> MAFISSGYNPEKPMANRITDIGPRKFDEFFPPVIAKNFGSWLYHEILEPGVLMHVAESGDKVYTVRVGAARLMSITHIREMCDIADKYCGGHLRFTTRNNVEFMVADEASLKALKEDLASRKFDGGSLKFPIGGTGAGVSNIVHTQGWVHCHTPATDASGPVKAIMDEVFEDFQSMRLPAPVRISLACCINMCGAVHCSDIGVVGIHRKPPMIDHEWTDQLCEIPLAVASCPTAAVRPTKLEIGDKKVNTIAIKNERCMYCGNCYTMCPALPISDGEGDGVVIMVGGKVSNRISMPKFSKVVVAYIPNEPPRWPSLTKTIKHIIEVYSANAYKYERLGEWAERIGWERFFSLTG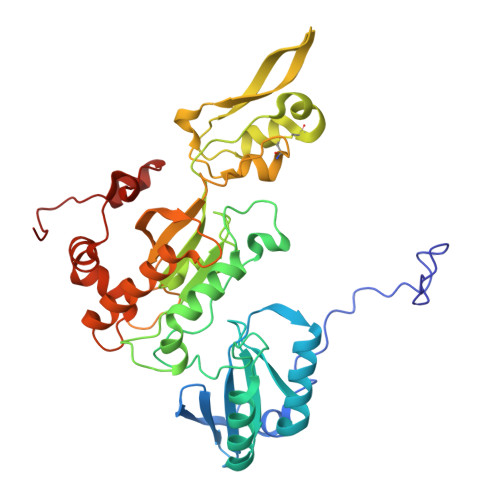LEFSHHLIDDFRDPAYYTWRQSTQFKF> Y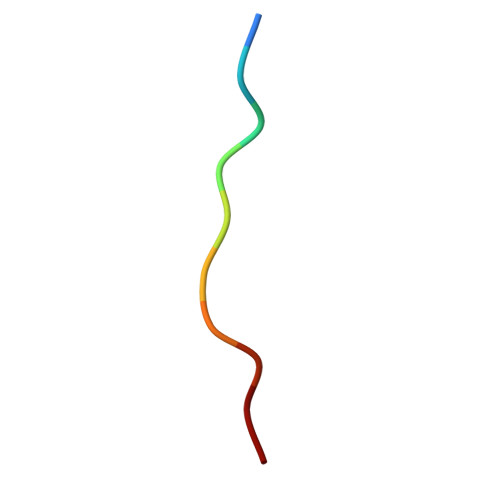VEPTAPQVL> SMTMINGYEQSDREEKIDILNLESLEKQAEEIIPAGGFGYIAGGSEDEWTLKQNRMAFHHRQIAPKALSGIEKPELNTEIFGIPLNTPVMMAPAGAQGLAHSQGE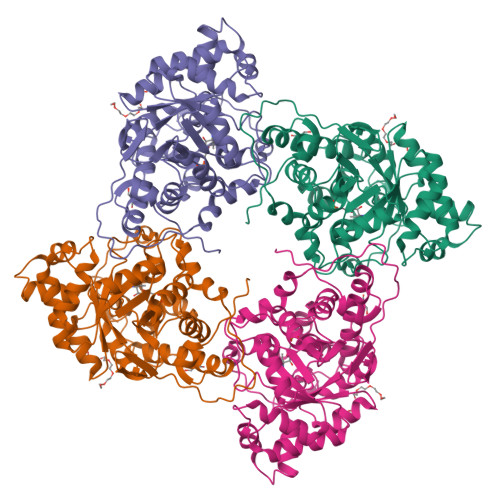KDTARGLAAVGGLMAQSTYSSVSIAETAAAGGDAPQFFQLYMSKDWNFNESLLDEAKKANVKAIILTVDATVDGYREADIKNKFTFPLPMANLIKFSEGNGQGKGIEEIYASAAQNIRPEDVKRIADYTNLPVIVKGIQTPEDAIRAIDAGAAGIYVSNHGGRQLNGGPASFDVLEDIATAVNKQVPIIFDSGVRRGSDVFKALASGADLVALGRPVIYGLALGGAKGVQSVFEHLNHELEIVMQLAGTKTIEDVKNNSLLNIKY>AAMVTQRFVELGWIDSTSPVNEQITNPALVEQIYHSNNDQLLWSDLATANHFEAQLEVIHRASFSPLFSRQLFALKSYRQQDRWHEYDVLATDTLLQYLSYAEQAPKVGIAWFFEGQLDQPLAPPSEEAQLALHMAIGNQSLARLMDEYTPQDPAYQQLLQAYQSLSSIEFNEVALYEQMERLKRPGDPLSHREALVQRLALVNLDTTSILNDVAYYDASLEKPIKQFQKMHGLQTDGVIGPQTMKWLNTSVTERLALLALNAERIRLWPTQQDSMIVVN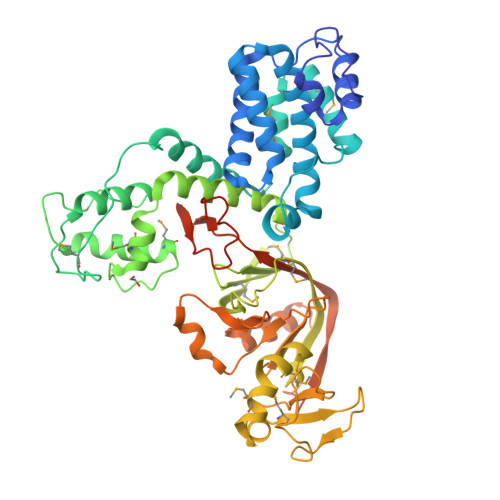VPGFDMKYWDAGREVFESKVVVGKTTRPTPVMNTKLDSLIINPTWNVPHKIMVEDILPMVKRDSEYLANHHMEIIRGWSDPEVIDPALIDWEAVEPETFPYRLRQQAGVQNALGTYKFNTPNSRAIYLHDTPSKHLFNNASRAFSSGCIRVENAEKFAQTLLANQGITLDDFPVSTQAIALKKRIPVHIIYQTVWYEEGVLHYRDDIYHYDALALGNGDASPNLTKIENLYFQGSSSHHHHHH[2x]>MEILYIKGDATAPIGSGVKVITHICNDIGGWGKGFVLALSKKWKMPEEAYRQWYKSQEEFTLGAVQFVNVENKLYVANMIGQHGIYKDSKGLPPIRYDAVRQCLKEVALFTIAHKASVHMPRIGCGLAGGKWELME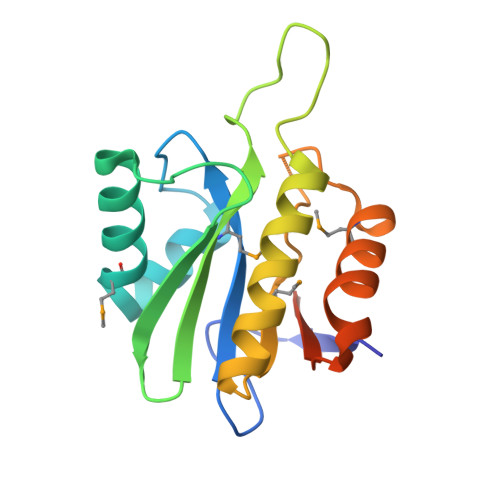QIIKEELITKEIAVTVYDLMAGDPLEHHHHHH[2x]> APSPIIKFPGDVAPKTDKELAVQYLNTFYGCPKESCNLFVLKDTLKKMQKFFGLPQTGDLDQNTIETMRKPRCGNPDVANYNFFPRKPKWDKNQITYRIIGYTPDLDPETVDDAFARAFQVWSDVTPLRFSRIHDGEADIMINFGRWEHGDGYPFDGKDGLLAHAFAPGTGVGGDSHFDDDELWTLGEGQVVRVKYGNADGEYCKFPFLFNGKEYNSCTDTGRSDGFLWCSTTYNFEKDGKYGFCPHEALFTMGGNAEGQPCKFPFRFQGTSYDSCTTEGRTDGYRWCGTTEDYDRDKKYGFCPETAMSTVGGNSEGAPCVFPFTFLGNKYESCTSAGRSDGKMWCATTANYDDDRKWGFCPDQGYSLFLVAAHAFGHAMGLEHSQDPGALMAPIYTYTKNFRLSQDDIKGIQELYGASPDIDLGTGPTPTLGPVTPEICKQDIVFDG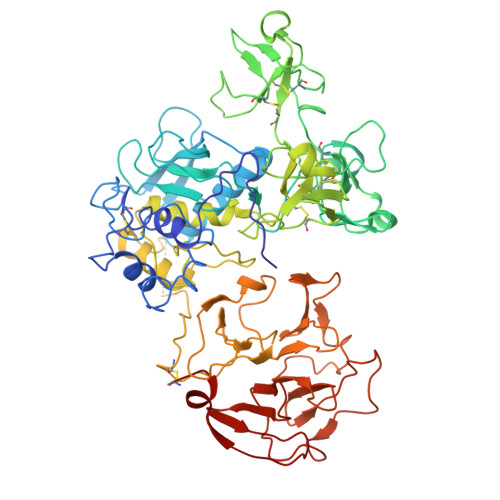IAQIRGEIFFFKDRFIWRTVTPRDKPMGPLLVATFWPELPEKIDAVYEAPQEEKAVFFAGNEYWIYSASTLERGYPKPLTSLGLPPDVQRVDAAFNWSKNKKTYIFAGDKFWRYNEVKKKMDPGFPKLIADAWNAIPDNLDAVVDLQGGGHSYFFKGAYYLKLENQSLKSVKFGSIKSDWLGC> MAKVSLEKDKIKFLLVEGVHQKALESLRAAGYTNIEFHKGALDDEQLKESIRDAHFIGLRSRTHLTEDVINAAEKLVAIGAFAIGTNQVDLDAAAKRGIPVFNAPFSNTRSVAELVIGELLLLLRGVPEANAKAHRGVWNKLAAGSFEARGKKLGIIGYGHIGTQLGILAESLGMYV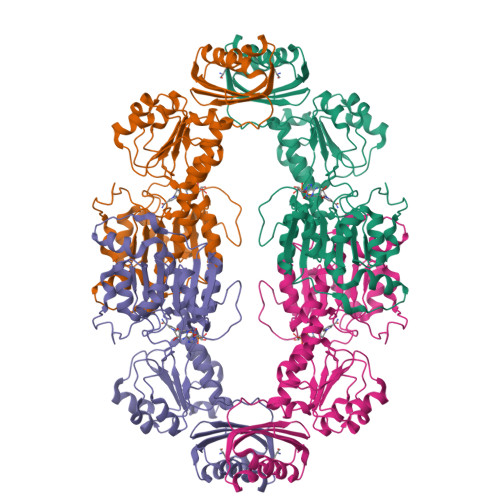YFYDIENKLPLGNATQVQHLSDLLNMSDVVSLHVPENPSTKNMMGAKEISLMKPGSLLINASRGTVVDIPALADALASKHLAGAAIDVFPTEPATNSDPFTSPLAEFDNVLLTPHIGGSTQEAQENIGLEVAGKLIKYSDNGSTLSAVNFPEVSLPLHVGRRLMHIHENRPGVLTALNKIFAEQGVNIAAQYLQTSAQMGYVVIDIEADEDVAEKALQAMKAIPGTIRARLLY(4S)-imidazolidine-4-carbonitrile | C4 H7 N3 | 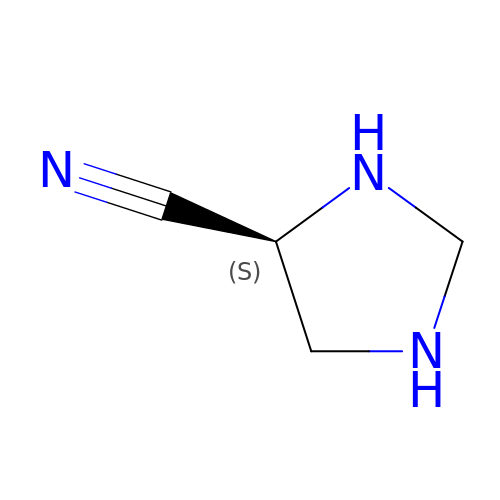FEQLHIQTBHWUKN-UHFFFAOYSA-N> MTPPHNYLAVIKVVGIGGGGVNAVNRMIEQGLKGVEFIAINTDAQALLMSDADVKLDVGRDSTRGLGAGADPEVGRKAAEDAKDEIEELLRGADMVLVTAGEGGGTGTGGAPVVASIARKLGALTVGVVTRPFSFEGKRRSNQAENGIAALRESCDTLIVIPNDRLLQMGDAAVSLMDAFRSADEVLLNGVQGITDLITTPGLINVDFADVKGIMSGAGT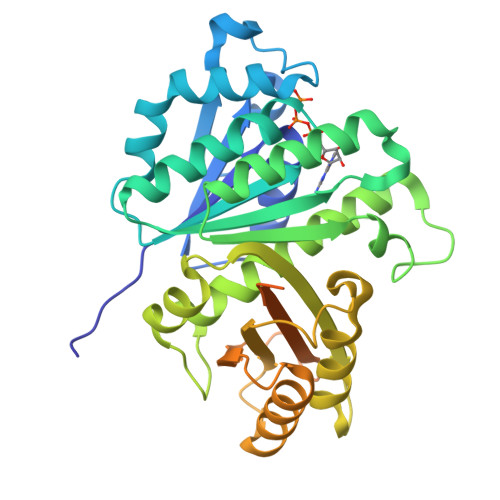ALMGIGSARGEGRSLKAAEIAINSPLLEASMEGAQGVLMSIAGGSDLGLFEINEAASLVQDAAHPDANIIFGTVIDDSLGDEVRVTVIAAGFDVSGPGRKPVMGETGGAHRIESAKAGKLTSTLFEPVDAVSVPLHTNGATLSIGGDDDDVDVPPFMRR>[2x]SNAMKIGIIGAMEQEVAILKDKIEGLSTVTKAGCTFYT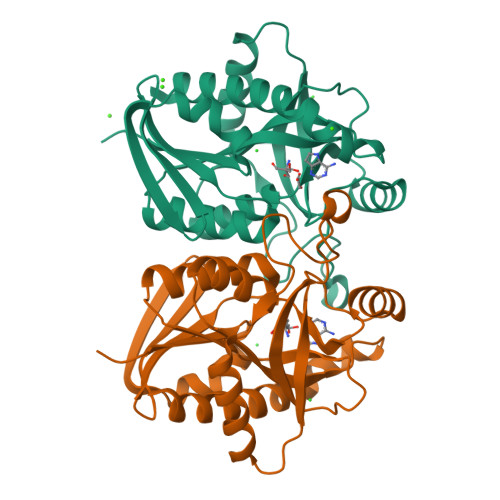GTLNGADVVLLQSGIGKVAAAVGTTLLIAEHNVDVVLNTGSAGGFDSSLNLGDVVISTEVRHHDADVTAFGYEMGQMAQQPAAFIADEKLITTAEQALTEMSDKHAVRGLICTGDVFVCTPERQEFIRTHFPSVIAVEMEASAIAQTCHQFNTPFVVVRAISDVADKESPMSFDEFLPLAAQSSSEMVLNMVTLLK>MRIVPFGAAREVTGSAHLLLAGGRRVLLDCGMFQGKEEARNHAPFGFDPKEVDAVLLTHAHLDHVGRLPKLFREGYRGPVYATRATVLLMEIVLEDALKVMDEPFFGPEDVEEALGHLRPLEYGEWLRLGALSLAFGQAGHLPGSAFVVAQGEGRTLVYSGDLGNREKDVLPDPSLPPLADLVLAEGTYGDRPHRPYRETVREFLEILEKTLSQGGKVLIPTFAVERAQEILYVLYTHGHRLPRAPIYLDSPMAGRVLSLYPRLVRYFSEEVQAHFLQGKNPFRPAGLEVVEHTEASKALNRAPGPMVVLAGSGMLAGGRILHHLKHGLSDPRNALVFVGYQPQGGLGAEIIA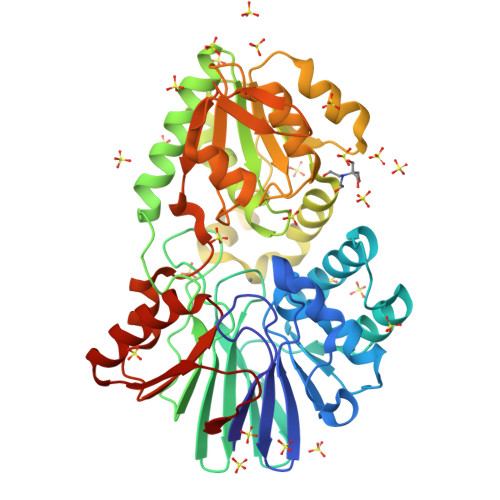RPPAVRILGEEVPLRASVHTLGGFSGHAGQDELLDWLQGEPRVVLVVGEEEKLLALGKLLALRGQEVSLARFGEGVPV[4x]> KQPPSNPPP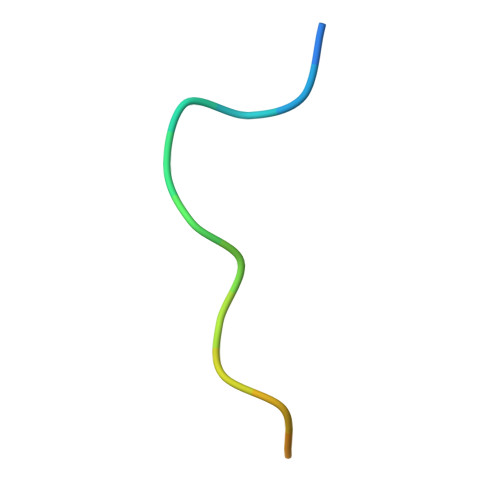RPPAEARKK> DIYCYEEF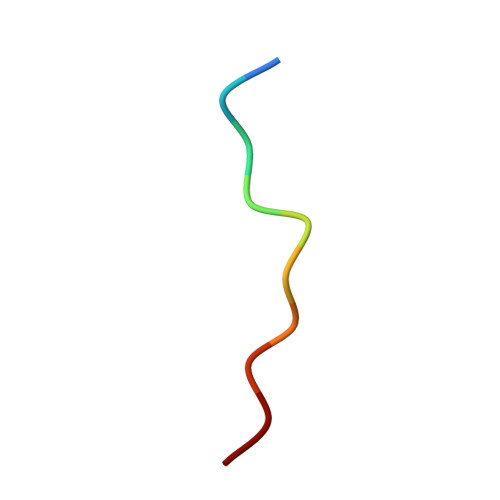SD>MKGPAFEFAVAMMKRNASTVKTEYGEFTMLGIYDRWAVLPRHAKPGPTILMNDQEVGVLDAKELVDKDGTNLELTLLKLNRNEKFRDIRGFLAREEVEVNEAVLAINTSKFPNMYIPVGQVTDYGFLNLGGTPTKRMLVYNFPTRAGQCGGVLMSTGKVLGIHVGGNGHQGFSAALLRHYFNEEQHHHHHH[2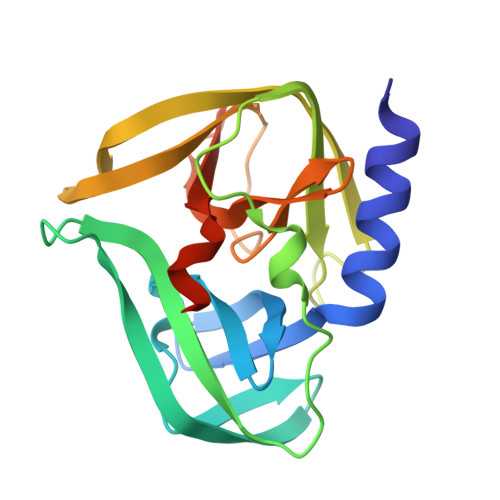x]> MRGSHHHHHHGSELSKSSIVDKVELDHTTLYQGEMTSIKVSFSDKENQKIKPGDTITLTLPDALVGMTENDSSPRKINLNGLGEVFIYKDHVVATFNEKVESLHNVNGHFSFGIKTLITNSSQPNVIETDFGTATATQRLTIEGVTNTETGQIERDYPFFYKVGDLAGESNQVRWFLNVNLNKSDVTEDISIADRQG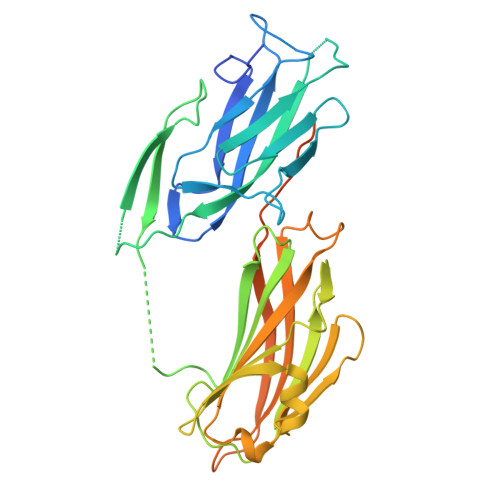SGQQLNKESFTFDIVNDKETKYISLAEFEQQGYGKIDFVTDNDFNLRFYRDKARFTSFIVRYTSTITEAGQHQATFENSYDINYQLNNQDATNEKNTSQVKNVFVEGEASGNQNVEMPTEESLDIPLETIDEWEPKTPTSEQATETSEKTD> GSPGISGGGGGILDSMGRLENLGRIQFSVGYNFQESTLTVKVMKAQELPAKDFSGTSDPFVKIYLLPDKKHK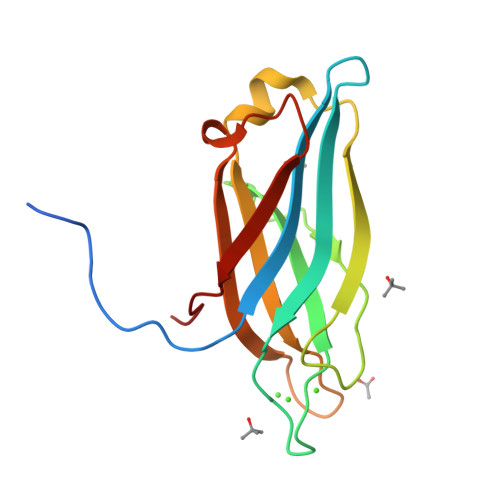LETKVKRKNLNPHWNETFLFEGFPYEKVVQRILYLQVLDYDRFSRNDPIGEVSIPLNKVDLTQMQTFWKDLKPCSD>[12x]SYSSIKLSNNNNNSNSNN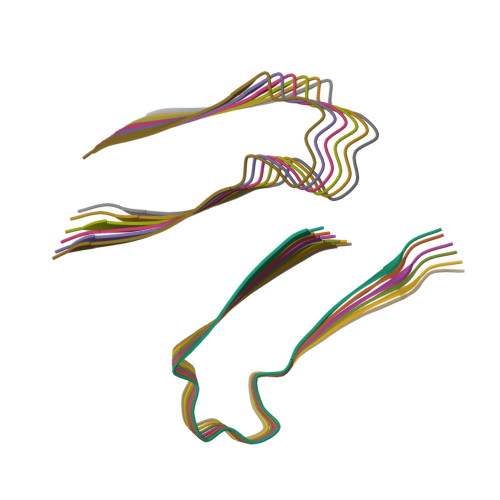IEISKSESCNASDIGGTNNNNASRTIASAAVGEETSTLSSTSHEHNNNPNNDT>GP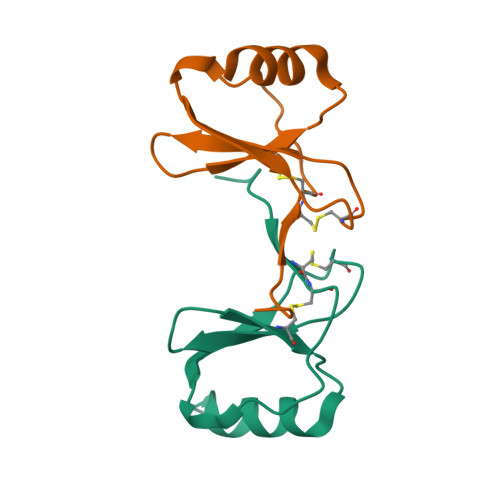YHPSECCFTYTTYKIPRQRIMDYYETNSQCSKPGIVFITKRGHSVCTNPSDKWVQDYIKDMKEN[4x]> MERNKLARQIIDTCLEMTRLGLNQGTAGNVSVRYQDGMLITPTGIPYEKLTESHIVFIDGNGKHEEGKLPSSSWRFHMAAYQSRPDANAVVHNHAVHCTAVSILNRSIPAIHYMIAAAGGNSIPCAPYATFGTRELSEHVALALKNRKATLLQHHGLIACEVNLEKALWLAHEVEVLAQLYL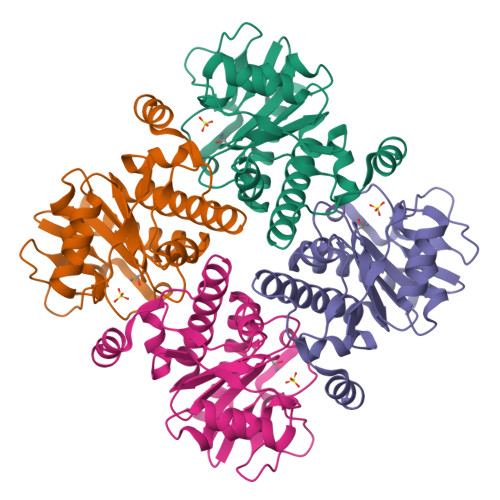TTLAITDPVPVLSDEEIAVVLEKFKTYGLRIEE> GSTREPEIASSLIKQIFSHYVKTPVTRDAYKIVEKCSERYFKQISSDLEAYSQHAGRKTVEMADVELLMRRQGLVTDKMPLHVLVERHLPLEYRKLLIPIAVSGNKVIPCK;> GRRTV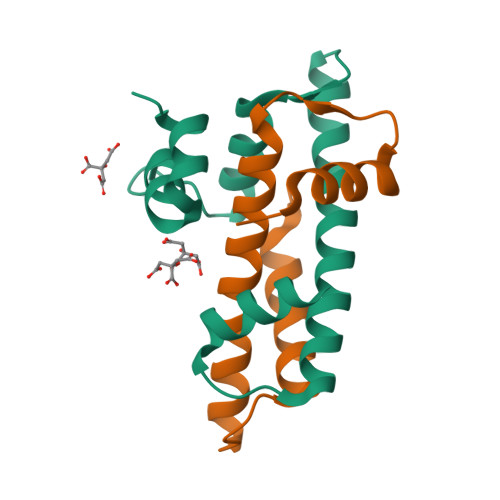PRGTLRKIIKKHKPHLRLAANTDLLVHLSFLLFLHRLAEEARTNAFENKSKIIKPEHTIAAAKVILKKSRG Bacterial HSS is mostly found in α-proteobacteria and in some β- and γ-proteobacteria, including pathogenic strains such as Legionella pneumophila, Brucella spp. and various P. aeruginosa strains, including PA7 and PA14. It catalyzes the conversion of two molecules of putrescine (PUT; 1,4-diaminobutane) into one molecule of sym-homospermidine [HSP; bis(4-aminobutyl)amine] as the main reaction along with several side reactions (Ober et al., 1996; Böttcher et al., 1994). Bacterial HSS is NAD+-dependent, active at neutral to basic pH with an optimum at pH ∼8.8, and shows increased activity in the presence of 50 mM potassium ion. BvHSS forms a dimer, with each subunit containing a boot-shaped substrate-binding pocket between an NAD(P)-binding Rossmann-like domain and an HSS-like domain. The cofactor NAD+ is bound as a prosthetic group in the binding pocket with its nicotinamide ring being part of the active site.

To experimentally substantiate this interaction, the tryptophan residue was exchanged for residues with reduced aromatic character (W229F, W229Y and W229H), for both acidic (W229E) and basic (W229K) residues and for alanine (W229A). Except for the W229F and W229Y variants, which retained very low activity (∼2% and 1% of the wild-type activity, respectively), all other variants were inactive. In conclusion, the decreased or abolished activity should be caused by the exchange of Trp229 and not by structural perturbation of the binding pocket. In the W229F variant, the location of the Phe229 phenyl ring is distinctly defined by the electron-density distribution. Consequently, the reduced activity of the variant is not caused by obstruction of the active site due to an inappropriately orientated phenyl ring. In the structure of the W229F variant, the side chain of the variant residue Phe229 sterically confines the active site to similar spatial dimensions as in wild-type BvHSS. In conclusion, we suggest the weaker cation–π interaction in the W229F and W229Y variants to be the reason for their reduced activities as explained in the following. Firstly, the Phe229 benzene moiety is shifted in relation to the Trp229 benzene moiety and therefore also in relation to the ‘center amino site’. The resulting cation–π interaction geometry in the W229F variant would consistently be more off-centered and therefore energetically less favored. Secondly, the phenyl ring (and similarly the phenol ring in the W229Y variant) exhibits less negative electrostatic potential and a smaller size of its π-electron system compared with the indole ring, resulting in a smaller cation–π interaction energy.

>GPMGTDWPVYHRIDGPIVMIGFGSIGRGTLPLIERHFAFDRSKLVVIDPSDEARKLAEARGVRFIQQAVTRDNYRELLVPLLTAGPGQGFCVNLSVDTSSLDIMELARENGALYIDTVVEPWLGFYFDPDLKPEARSNYALRETVLAARRNKPGGTTAVSCCGANPGMVSWFVKQALVNLAADLGVTGEEPTTREEWARLAMDLGVKGIHIAERDTQRASFPKPFDVFVNTFSVEGFVSEGLQPAELGWGTFERWMPDNARGHDSGCGAGIYLLQPGANTRVRSWTPTAMAQYGFLVTHNESISIADFLTVRDAAGQAVYRPTCHYAYHPCNDAVLSLHEMFGSGKRQSDWRILDETEIVDGIDELGVLLYGHGKNAYWYGSQLSIEETRRIAPDQNATGLQVSSAVLAGMVWALENPNAGIVEADDLDFRRCLEVQTPYLGPVVGVYTDWTPLAGRPGLFPEDIDTSDPWQFRNVLVRD[2x]>[12x]GGEVPIGDPKELNGMEIAAVYLQPIEMEPRGIDLAASLADIHLEADIHALKNNPNGFPEGFWMPYLTIAYELKNTDTGAIKRGTLMPMVA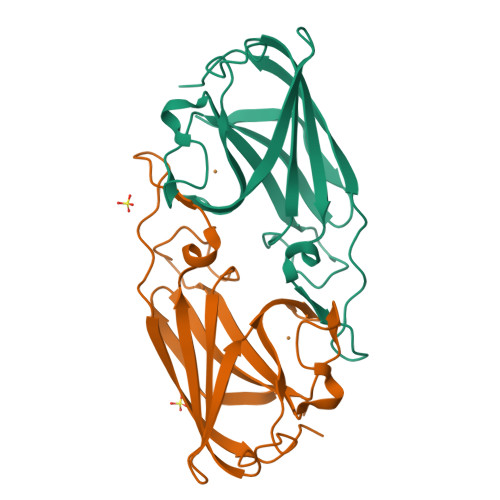DHGPHYGANIAMEKDKKGGFGVGNYELTFYISNPEKQGFGRHVDEETGVGKWFEPFKVDYKFKYTGTPK>MQSSVNEFLTPRHIDVQVVSQTRAKITLEPLERGFGHTLGNALRRILLSSMPGCAVVEAEIDGVLHEYSAIEGVQEDVIEILLNLKGLAIKLHGRDEVTLTLAKKGSGVVTAADIQLDHDVEIINGDHVIANLADNGALNMKLKVARGRGYEPADARQSDEDESRSIGRLQLDASFSPVRRVSYVVENARVEQRTNLDKLVLDLETNGTLDPEEAIRRAATILQQQLAAFVDLKGDSEPVVEEQEDEIDPILLRPVDDLELTVRSANCLKAENIYYIGDLIQRTEVELLKTPNLGKKSLTEIKDVLASRGLSLGMRLDNWPPASLKKDDKATA[2x];> MAYSYTEKKRIRKDFSKLPDVMDVPYLLAIQLDSYREFLQAGATKEQFRDVGLHAAFKSVFPIISYSGNAALEYVGYRLGEPAFDVKECVLRGVTFAVPLRVKVRLIIFDRESSNKAIKDIKEQEVYMGEIPLMTENGTFIINGTERVIVSQLHRSPGVFFDHDRGKTHSSGKLLYSARIIPYRGSWLDFEFDPKDCVFVRIDRRRKLPASVLLRALGYSTEEILNAFYATNVFHIKGETLNLELVPQRLRGEVASIDIKDGSGKVIVEQGRRITARHINQLEKAGVSQLEVPFDYLIGRTIAKAIVHPATGEIIAECNTELTLDLLAKVAKAQVVRIETLYTNDIDCGPFISDTLKIDNTSNQLEALVEIYRMMRPGEPPTKEAAETLFGNLFFSAERYDLSAVGRMKFNRRIGRTEIEGPGVLSKEDIIDVLKTLVDIRNGKGIVDDIDHLGNRRVRCVGEMAENQFRVGLVRVERAVKERLSMAESEGLMPQDLINAKPVAAAIKEFFGSSQLSQFMDQNNPLSEITHKRRVSALGPGGLTRERAGFEVRDVHPTHYGRVCPIETPEGPNIGLINSLATYARTNKYGFLESPYRVVKDSLVTDEIVFLSAIEEADHVIAQASATLNEKGQLVDELVAVRHLNEFTVKAPEDVTLMDVSPKQVVSVAASLIPFLEHDDANRALMGSNMQRQAVPTLRADKPLVGTGMERNVARDSGVCVVARRGGVIDSVDASRVVVRVADDEVETGEAGVDIYNLTKYTRSNQNTCINQRPLVSKGDVVARGDILADGPSTDMGELALGQNMRVAFMPWNGFNFEDSICLSERVVQEDRFTTIHIQELTCVARDTKLGPEEITADIPNVGEAALNKLDEAGIVYVGAEVQAGDILVGKVTPKGETQLTPEEKLLRAIFGEKASDVKDTSLRVPTGTKGTVIDVQVFTRDGVERDSRALSIEKMQLDQIRKDLNEEFRIVEGATFERLRAALVGAKAEGGPALKKGTEITDDYLDGLERGQWFKLRMADDALNEQLEKAQAYISDRRQLLDDKFEDKKRKLQQGDDLAPGVLKIVKVYLAIKRRIQPGDKMAGRHGNKGVVSVIMPVEDMPHDANGTPVDIVLNPLGVPSRMNVGQILETHLGLAAKGLGEKINRMLEEQRKVAELRKFLHEIYNEIGGREENLDELGDNEILALAKNLRGGVPMATPVFDGAKEREIKAMLKLADLPESGQMRLFDGRTGNQFERPTTVGYMYMLKLNHLVDDKMHARSTGSYSLVTQQPLGGKAQFGGQRFGEMEVWALEAYGAAYTLQEMLTVKSDDVNGRTKMYKNIVDGDHRMEAGMPESFNVLIKEIRSLGIDIELETE;> MKDLLNLLKNQGQIEEFDAIRIGLASPEMIRSWSFGEVKKPETINYRTFKPERDGLFCAKIFGPVKDYECLCGKYKRLKHRGVICEKCGVEVALAKVRRERMGHIELASPVAHIWFLKSLPSRIGLLLDMTLRDIERVLYFESYVVIDPGMTTLEKGQLLNDEQYFEALEEFGDDFDARMGAEAVHELLNAIDLEHEIGRLREEIPQTNSETKIKKLSKRLKLMEAFQGSGNKPEWMVLTVLPVLPPDLRPLVPLDGGRFATSDLNDLYRRVINRNNRLKRLLDLAAPDIIVRNEKRMLQEAVDALLDNGRRGRAITGSNKRPLKSLADMIKGKQGRFRQNLLGKRVDYSGRSVITVGPTLRLHQCGLPKKMALELFKPFIFGKLEGRGMATTIKAAKKMVERELPEVWDVLAEVIREHPVLLNRAPTLHRLGIQAFEPVLIEGKAIQLHPLVCAAYNADFDGDQMAVHVPLTLEAQLEARALMMSTNNILSPANGEPIIVPSQDVVMGLYYMTREAINAKGEGMAFADLQEVDRAYRSGQASLHARVKVRINEKIKGEDGQLTANTRIVDTTVGRALLFQVVPAGLPFDVVNQSMKKKAISKLINHCYRVVGLKDTVIFADQLMYTGFAYSTISGVSIGVNDFVIPDEKARIINAATDEVKEIESQYASGLVTQGEKYNKVIDLWSKANDEVSKAMMANLSKEKVVDREGKEVDQESFNSMYMMADSGARGSAAQIRQLAGMRGLMAKPDGSIIETPITANFREGLNVLQYFISTHGARKGLADTALKTANSGYLTRRLVDVAQDLVVTEIDCGTEHGLLMSPHIEGGDVVEPLGERVLGRVIARDVFKPGSDEVIVPAGTLIDEKWVDFLEVMSVDEVVVRSPITCETRHGICAMCYGRDLARGHRVNIGEAVGVIAAQSIGEPGTQLTMRTFHIGGAASRTSAADNVQVKNGGTIRLHNLKHVVRADGALVAVSRSGELAVADDFGRERERYKLPYGAVISVKEGDKVDPGAIVAKWDPHTHPIVTEVDGTVAFVGMEEGITVKRQTDELTGLTNIEVMDPKDRPAAGKDIRPAVKLIDAAGKDLLLPGTDVPAQYFLPANALVNLTDGAKVSIGDVVARIPQETSKTRDITGGLPRVADLFEARRPKEPSILAEISGTISFGKETKGKRRLVITPNDGSDPYEELIPKWRHLNVFEGEQVNRGEVISDGPSNPHDILRLLGVSSLAKYIVNEIQDVYRLQGVKINDKHIETILRQMLRKVEVSESGDSSFIKGDQVELTQVLEENEQLGTEDKFPAKYERVLLGITKASLSTESFISAASFQETTRVLTEAAVTGKRDFLRGLKENVVVGRLIPAGTGLAYHSERKRQRDLGKPQRVSASE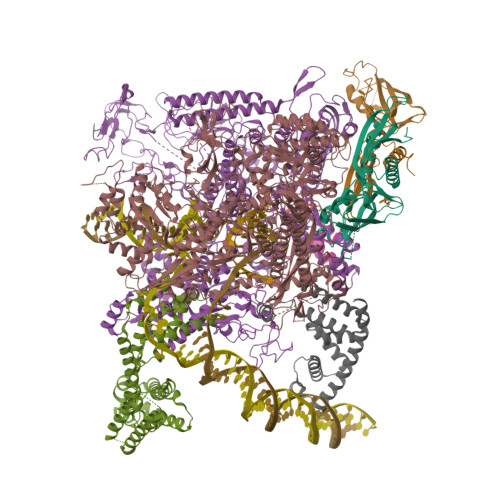AEAALTEALNSSGN;> MARVTVEDCLDNVDNRFELVMLATKRARQLATGGKEPKVAWENDKPTVVALREIASGLVDENVVQQEDIVEDEPLFAAFDDEANTEAL;> MSGKAQQQSRLKELIARGREQGYLTYAEVNDHLPEDISDPEQVEDIIRMINDMGINVFETAPDADALLLAEADTDEAAAEEAAAALAAVESDIGRTTDPVRMYMREMGTVELLTREGEIEIAKRIEEGIREVMSAIAQFPGTVDSILADYNRIVAEGGRLSDVLSGYIDPDDGSLPAEEVEPVNLKDDSADSKEKDDEEEESDDSSDSDDEGDGGPDPEEARLRFTAVSEQLDKAKKALKKHGRGSKQATAELTGLAELFMPIKLVPKQFDALVARVRSALEGVRAQERAIMQLCVRDARMPRADFLRLFPNHETDEKWVDSVLKSKPKYAEAIERLRDDILRNQQKLAALESEVELTVAEIKEINRAMSIGEAKARRAKKEMVEANLRLVISIAKKYTNRGLQFLDLIQEGNIGLMKAVDKFEYRRGYKFSTYATWWIRQAITRSIADQARTIRIPVHMIETINKLNRISRQMLQEMGREPTPEELGERMDMPEDKIRKVLKIAKEPISMETPIGDDEDSHLGDFIEDSTMQSPIEMATSESLKESTREVLAGLTAREAKVLRMRFGIDMNTDHTLEEVGKQFDVTRERIRQIEAKALRKLRHPSRSEHLRSFLDE;> MFQSTEQALAVAYWMFEQQPGPRSSTAMVIDSLRERFDRRFIERLPSGLSPHEWQAQAVMTVRFAQRQLAAHPLELAVVRAEFARGRDFVLGLAALRDWLKPAAGPIEQRAALALLMRMFRRPPSSIREIERLSGLSKSTLHRWDKEWRERVAALLRQALLRLEEPMAQVGIVCEH>MENTENSVDSKSIKNLEPKIIHGSESMDSGISLDNSYKMDYPEMGLCIIINNKNFHKSTGMTSRSGTDVDAANLRETFRNLKYEVRNKNDLTREEIVELMRDVSKEDHSKRSSFVCVLLSHGEAGIIFGTNGPVDLKKITNFFRGDRCRSLTGKPKLFIIQACRGTELDCGIETDSGVDDDMACHKIPVEADFLYAYSTAPGYYSWRNSKDGSWFIQSLCAMLKQYADKLEFMHILTRVNRKVATEFESFSFDATFHAKKQIPCIHS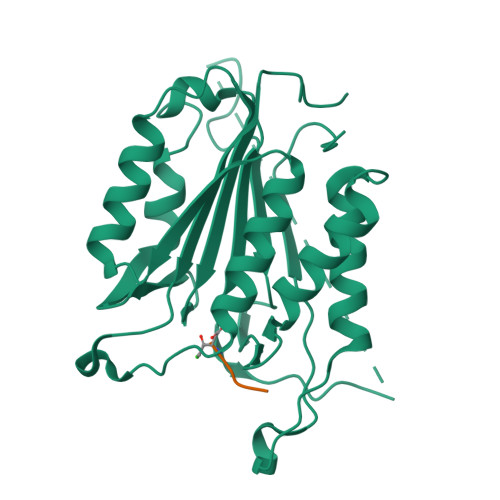MLTKELYFYH[2x]>[8x]HHHHHHSSGLGVLFQGPGSKDFQGMLEYKREDEQKLVKNLILELKPRGVAVNLIPGLPAYILFMCVRHADYLNDDQKVRSLL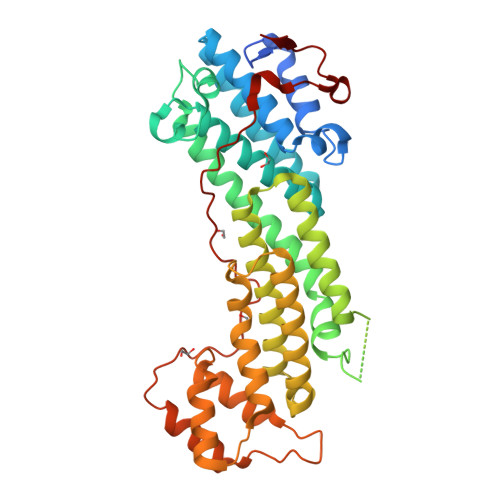TSTINSIKKVLKKRGDDFETVSFWLSNTCRFLHCLKQYSGEEGFMKHNTSRQNEHCLTNFDLAEYRQVLSDLAIQIYQQLVRVLENILQPMIVSGMLEHETIQGVSGVKPTGLRKRTSSIADEGTYTLDSILRQLNSFHSVMCQHGMDPELIKQVVKQMFYIVGAITLNNLLLRKDMCSWSKGMQIRYNVSQLEEWLRDKNLMNSGAKETLEPLIQAAQLLQVKKKTDDDAEAICSMCNALTTAQIVKVLNLYTPVNEFEERVSVSFIRTIQMRLRDRKDSPQLLMDAKHIFPVTFPFNPSSLALETIQIPASLGLGFIARV>MRVAMISMHTSPLQQPGTGDSGGMNVYILSTATELAKQGIEVDIYTRATRPSQGEIVRVAENLRVINIAAGPYEGLSKEELPTQLA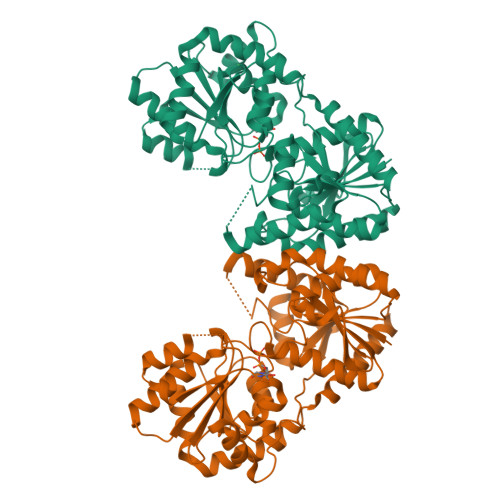AFTGGMLSFTRREKVTYDLIHSHYWLSGQVGWLLRDLWRIPLIHTAHTLAAVKNSYRDDSDTPESEARRICEQQLVDNADVLAVNTQEEMQDLMHHYDADPDRISVVSPGADVELYSPGNDRATERSRRELGIPLHTKVVAFVGRLQPFKGPQVLIKAVAALFDRDPDRNLRVIICGGPSGPNATPDTYRHMAEELGVEKRIRFLDPRPPSELVAVYRAADIVAVPSFNESFGLVAMEAQASGTPVIAARVGGLPIAVAEGETGLLVDGHSPHAWADALATLLDDDETRIRMGEDAVEHARTFSWAATAAQLSSLYNDAIANENVDGETHHGLEHHHHHH[2x]5'-{[(2R,4R)-1-{2-[(2-amino-7,7-dimethyl-4-oxo-3,4,7,8-tetrahydropteridine-6-carbonyl)amino]ethyl}-2-carboxypiperidin-4-yl]sulfonyl}-5'-deoxyadenosine 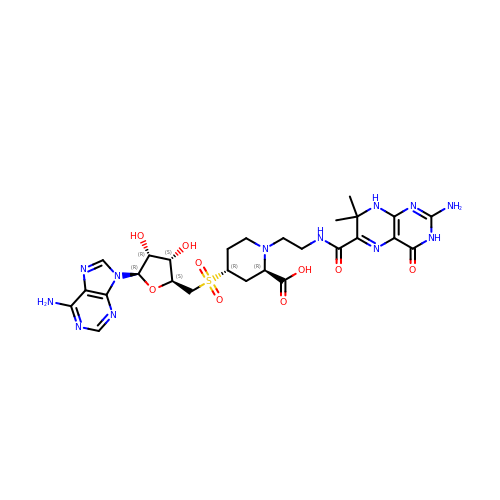| C27 H36 N12 O9 S | LIEKVCRXNQELKW-NERDUYAPSA-N>GHMAKQYDSVECPFCDEVSKYEKLAKIGQGTFGEVFKARHRKTGQKVALKKVLMENEKEGFPITALREIKILQLLKHENVVNLIEICRTKASPYNRCKGSIYLVFDFCEHDLAGLLSNVLVKFTLSEIKRVMQMLLNGLYYIHRNKILHRDMKAANVLITRDGVLKLADFGLARAFSLAKNSQPNRYTNRVVTLWYRPPELLLGERDYGPPIDLWGAGCIMAEMWTRSPIMQGNTEQHQLALISQLCGSITPEVWPNVDNYELYEKLELVKGQKRKVKDRLKAYVRDPYALDLIDKLLVLDPAQRIDSDDALNHDFFWSDPMPSDLKGMLST[3x];>MEGERKNNNKRWYFTREQLENSPSRRFGVDPDKELSYRQQAANLLQDMGQRLNVSQLTINTAIVYMHRFYMIQSFTQFPGNSVAPAALFLAAKVEEQPKKLEHVIKVAHTCLHPQESLPDTRSEAYLQQVQDLVILESIILQTLGFELTIDHPHTHVVKCTQLVRASKDLAQTSYFMATNSLHLTTFSLQYTPPVVACVCIHLACKWSNWEIPVSTDGKHWWEYVDATVTLELLDELTHEFLQILEKTPNRLKRIWNWRACEAA[3x];>SNANREDRNVLRMKERERRNQEIQQGEDAFPPSSPLFAEPYKVTSKEDKLSSRIQSMLGNYDEMKDFIGDRSIPK[3x];>XMEPVDPRLEPWKHPGSQPKTACTNCYCKKCCFHCQVCFITKALGISYGRKKRRQRRR[3x]

The HIV Tat protein bound to a host super elongation complex (SEC) recognizes TAR and releases the paused polymerase. HIV Tat binds simultaneously to TAR and positive elongation factor b (P-TEFb), composed of CDK9 and Cyclin T1 (CycT1) subunits. In turn, P-TEFb and the transcriptional elongation factors ELL2 and ENL/AF9 associate with hydrophobic segments in the approximately 1200-amino-acid AFF1 or AFF4 scaffold, together forming the SEC. P-TEFb triggers promoter escape by phosphorylating two negative elongation factors (DSIF and NELF), as well as the C-terminal domain (CTD) of Pol II.

To define the structural basis for the increased affinity of the AFF4-P-TEFb complex for Tat, we determined the crystal structure of the quaternary complex of P-TEFb with AFF42–73 and Tat1–57. Tat and AFF4 bind adjacent to each other on the CycT1 surface. AFF4 residues 34- to 69-fold on the CycT1 surface, making multiple direct contacts with Tat K28, F32, and E2 and burying Tat M1. The nexus of the Tat–AFF4 interface, Tat K28, is partially buried in a hydrophobic pocket formed by the side chains of AFF4 M62, F65, and Tat F32, and the main chain of AFF4 helix 2, residues 59–63. The Tat K28 side-chain amino group forms a hydrogen bond with the AFF4 E61 main-chain carbonyl at the pocket edge facing the solvent. Compared to the AFF4-P-TEFb complex, AFF4 structural segments in the Tat-AFF4-P-TEFb complex undergo unanticipated 1–2 Å backbone shifts to avoid unfavorable close contacts with Tat. In contrast to the Tat-P-TEFb complex, in which the CycT1 TRM is disordered between residues 253 and 260, this functionally important segment is ordered in two conformations in the Tat-AFF4-P-TEFb complex. CycT1 residues 253–259 loop over Tat helix 28–33 in two conformations that converge at CycT1 C261. C261 binds the shared Tat Zn2+ ion in all three complexes. In all complexes, W256 makes buried contacts with AFF4.> MRRLKGTIRHLD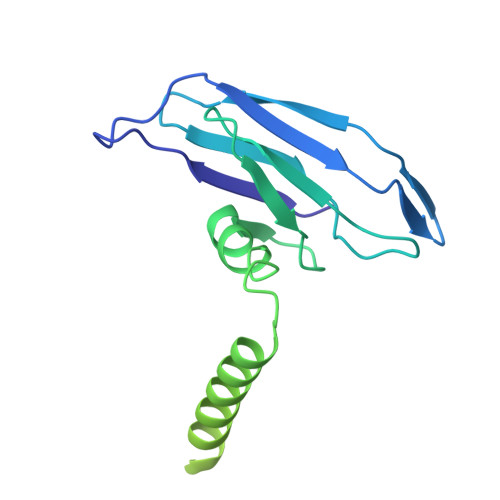DQPWINVSLFLTLINGTFNSANQYPIDTKHAKTDQNGEFVFNVVPNVGIDQSYYILTTPDNKKHSFTVPDGTSDIEFSVVREAGIIATDPEYTNVLNYLEDYIDDAIANIQASSVIAEIFTCGQTISALKALRFDSSTGKVFYASSSDATHLNKCVGVSSQSGVLNDNIQVVTSGYLSDQSWNWTIGSPIFFDSGGTLTHTPGSSYYQVIGIPVTTNKVLISVEQPIKL>[6x]MLNQELELSLNMAFARAREHRHEFMTVEHLLLALLSNPSAREALEACSVDLVALRQELEAFIEQTTPVLPASEEERDTQPTLSFQRVLQRAVFHVQSSGRNEVTGANVLVAIFSEQESQAAYLLRKHEVSRLDVVNFISHGTRKDEPTQSSDPGSQPNSEEQAGGEERTENFTTNLNQLARVGGIDPLIGREKELERAIQVLCRRRKNNPLLVGESGVGKTAIAEGLAWRIVQGDVPEVMADCTIYSLDIGSLLAGTKYRGDFEKRFKALLKQLEQDTNSILFIDEIHTIIGAGAASGGQVDAANLIKPLLSSGKIRVIGSTTYQEFSNIFEKDRALARRFQKIDITEPSIEETVQIINGLKPKYEAHHDVRYTAKAVRAAVELAVKYINDRHLPDKAIDVIDEAGARARLMPVSKRKKTVNVADIESVVARIARIPEKSVSQSDRDTLKNLGDRLKMLVFGQDKAIEALTEAIKMARAGLGHEHKPVGSFLFAGPTGVGKTEVTVQLSKALGIELLRFDMSEYMERHTVSRLIGAPPGYVGFDQGGLLTDAVIKHPHAVLLLDEIEKAHPDVFNILLQVMDNGTLTDNNGRKADFRNV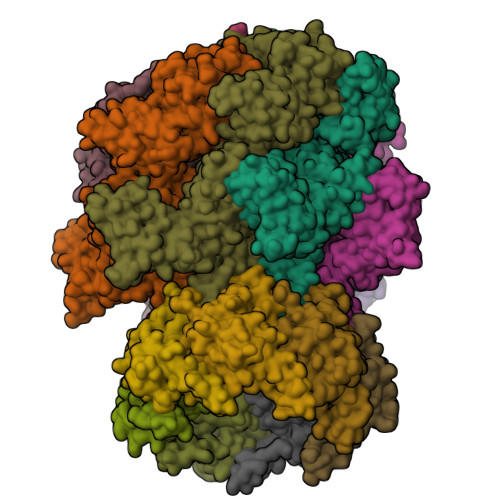VLVMTTNAGVRETERKSIGLIHQDNSTDAMEEIKKIFTPEFRNRLDNIIWFDHLSTDVIHQVVDKFIVELQVQLDQKGVSLEVSQEARNWLAEKGYDRAMGARPMARVIQDNLKKPLANELLFGSLVDGGQVTVALDKEKNELTYGFQSAQKHKAEAAH;>ALVPMVIEQTSRGERSFDIYSRLLKERVIFLTGQVEDHMANLIVAQMLFLEAENPEKDIYLYINSPGGVITAGMSIYDTMQFIKPDVSTICMGQAASMGAFLLTAGAKGKRFCLPNSRVMIHQPLGGYQGQATDIEIHAREILKVKGRMNELMALHTGQSLEQIERDTERDRFLSAPEAVEYGLVDSILTHRNRSHHHHHH[7x];> MGKTNDWLDFDQLAEEKVRDALKPPSMYKVILVNDDYTPMEFVIDVLQKFFSYDVERATQLMLAVHYQGKAICGVFTAEVAETKVAMVNKYARENEHPLLCTLEKA> GSHMLPSCKEDEYPVGSECCPKCSPGYRVKEACGELTGTVCEPCPPGTYIAHLNGL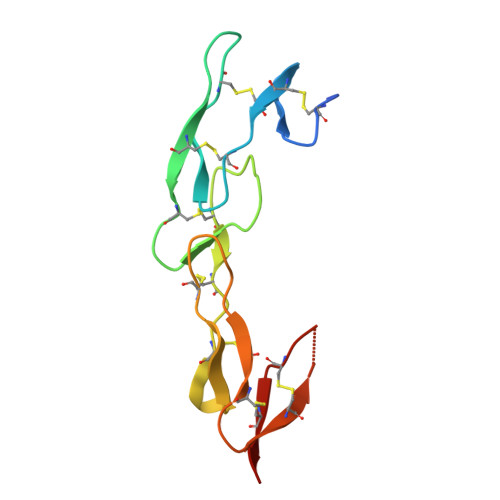SKCLQCQMCDPAMGLRASRNCSRTENAVCGCSPGHFCIVQDGDHCAACRAYA>[6x]MAGNKPFNKQQAEPRERDPQVAGLKVPPHSIEAEQSVLGGLMLDNERWDDVAERVVADDFYTRPHRHIFTEMARLQESGSPIDLITLAESLERQGQLDSVGGCAYLAELSKNTPSAANISAYADIVRERAVVREMISVANEIAEAGFDPQGRTSEDLLDLAESRVFKIAESRANKDEGPKNIADVLDATVARIEQLFQQPHDGVTGVNTGYDDLNKKTAGLQPSDLIIVAARPSMGKTTFAMNLVENAAMLQDKPVLIFSLEMPSEQIMMRSLASLSRVDQTKIRTGQLDDEDWARISGTMGILLEKRNIYIDDSSGLTPTEVRSRARRIAREHGGIGLIMIDYLQLMRVPALSDNRTLEIAEISRSLKALAKELNV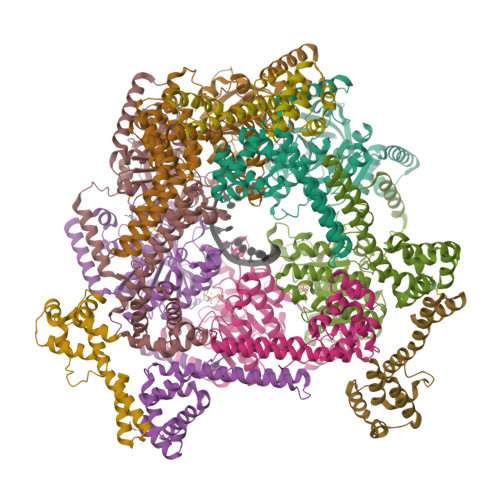PVVALSQLNRSLEQRADKRPVNSDLRESGSIEQDADLIMFIYRDEVYHENSDLKGIAEIIIGKQRNGPIGTVRLTFNGQWSRFDNYAGPQYDDE;>[3x]AAESGVSRPVPQLKRTTMRILIGLLVQNPELATLVPPLENLDENKLPGLGLFRELVNTCLSQPGLTTGQLLEHYRGTNNAATLEKLSMWDDIADKNIAEQTFTDSLNHMFDSLLELRQEELIARERTHGLSNEECLELWTLNQELAKK>AAEASKKPRQKRTATKAYNVTQAFGRRGPEQTQGNFGDQELIRQGTDYKHWPQIAQFAPSASAFFGMSRIGMEVTPSGTWLTYTGAIKLDDKDPNFKDQVILLNKHIDAYKTFP[6x]

The nucleocapsid (N) protein plays critical roles in coronavirus genome transcription and packaging, representing a key target for the development of novel antivirals, and for which structural information on ligand binding is scarce. The NTD is implicated in the binding and melting of regulatory elements required for transcription initiation, whereas the CTD drives protein dimerization and is thought to contribute to the binding of the RNA packaging signal (PS) sequence during virus particle assembly.

Complementary orthogonal biophysical methods, including isothermal titration calorimetry (ITC), 1H-saturation transfer difference (STD) and 1H15N-HSQC NMR experiments, further revealed that CA binds to the CTD. This was confirmed by the crystal structure of the CTD in complex with CA, determined at 1.7 Å resolution, which represents the first CTD structure bound to an exogenous small molecule. CA binds to a shallow pocket (volume of ~ 190 A3 ) formed between α-helices 1–2 and η-helix 2, close to the C-terminus. The CA molecule bound to one of the CTD protomers was unambiguously found by inspecting the 2Fo–Fc electron-density map. Nevertheless, this map only partially covers the CA aromatic ring most exposed to solvent. A close inspection of the structural complex shows that the binding of CA to the CTD is stabilized mainly by polar contacts of the carboxylate and carbonyl groups from CA’s tartarate and caffeoyl units, involving Arg276/Arg277 and three structural water molecules. The structure of the complex also shows one CA catechol ring laid inside a hydrophobic canyon formed by η-helix 2, α-helix 2 and the last two C-terminus residues (Phe363 and Pro364). When the apo and complexed structures were superposed, we observed no significant changes in the overall structures, as judged by the Cα RMSD (0.19 Å deviation). However, we noticed clear conformational changes in the side chains of Phe363, Pro364, Gln289 and Arg276, which contributed to the widening of the CA pocket. Arg276 had moved outwards, positioning its guanidine group at ideal distances to form electrostatic (NH1) and water-mediated (NH2) hydrogen-bond interactions with CA’s carboxylate group. Notably, the binding of CA to the CTD not only alters the topology but also the charge distribution of this region, which might explain why CA disrupts the N protein-RNA1 complex in solution.>[2x]NVIIGNQKLTINDVARVARNGTLVSLTNNTDILQGIQASCDYINNAVESGEPIFGVTSGFGGMANVAISREQASELQTNLVWFLKTGAGNKLPLADVRAAMLLRANSHMRGASGIRLELIKRMEIFLNAGVTPYVYEFGSIGASGDLVPLSYITGSLIGLDPSFKVDFNGKEMDAPTALRQLNLSPLTLLPKEGLAMMNGTSVMTGIAANCVYDTQILTAIAMGVHALDIQALNGTNQSFHPFIHNSKPHPGQLWAADQMISLLANSQLVRDELDGKHDYRDHELIQDRYSLRCLPQYLGPIVDGISQIAKQIEIEINSVTDNPLIDVDNQASYHGGNFLGQYVGMGMDHLRYYIGLLAKHLDVQIALLASPEFSNGLPPSLLGNRERKVNMGLKGLQICGNSIMPLLTFYGNSIADRFPTHAEQFNQNINSQGYTSATLARRSVDIFQNYVAIALMFGVQAVDLRTYKKTGHYDARASLSPATERLYSAVRHVVGQKPTSDRPYIWNDNEQGLDEHIARISADIAAGGVIVQAVQDIL

Enzymes with phenylalanine ammonia lyase (PAL) activity are able to catalyse non-oxidative deamination to yield cinnamate (1a) and ammonia from the proteinogenic amino acid L-phenylalanine (L-Phe, 2a). PALs also find use in the area of green chemistry and sustainable pharmaceutical manufacture as industrial biocatalysts, due to the reversibility of the deamination reaction. Although several crystal structures of PAL enzymes have been solved, none exists with the natural ligand trans-cinnamic acid bound in the active site, thereby preventing correct and unambiguous assignment of the phenylalanine-specific MIO-dependent ammonia lyase zymophore.

The gene encoding AvPAL was mutated, incorporating two surface substitutions (C503S and C565S, known to aid crystallisation) and replacement of the loop tyrosine with a catalytically inert but shape-complementary phenylalanine (Y78F). The triple variant was purified and co-crystallised with the natural deamination product. Superimposition of these two structures revealed excellent complementarity with a few small differences between the unoccupied and occupied active sites. The only backbone displacement was a shift in the outer active site loop, with the fully closed conformation from the previously reported structure seen to clash with the inner active site position 78 in the co-crystallised protein. In the case of the unoccupied enzyme, the amino acid at position 78 is tyrosine which points inward toward the active site, providing no contact with the outer loop, whereas the new structure features Y78F with a dihedral swing of ~140° causing the bulky side chain to protrude outwards. Other differences included H359 moving into the active site sphere in the cinnamate bound structure, along with smaller shifts in the positions of Q311 and R317 (SI). Presumably these represent movements which occur upon substrate binding, although they may be induced instead by the Y78F variation as exchange of polar and non-polar residues in the inner active site loop of related enzymes has been reported to influence conformational dynamics. Visualisation of the occupied active site allowed the identification of 19 residues within a 6 Å sphere of the ligand, including the MIO and catalytic amino acid at position 78, the carboxyl positioning residues, the hydrophobic aryl binding pocket and other assorted substrate-constraining side chains. The 19 amino acid active-site sequence motif, as inferred from the AvPAL-cinnamate structure, was used to distinguish potentially useful enzyme sequences from other family members.> MTTKEFEDTWAYNTIGSPFPDNPVRVKGQQNMYVALWYKFGKPIHGRAWNDNGNVECSFPYNKVELTGARDLGGQIQILTATEQDPTEQFKKTGFWYEWRPYKDRVNDQLLQLVRCGQSTPV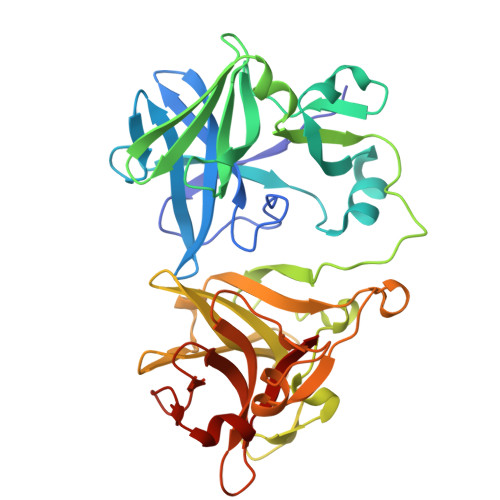IMKTKDGKDLLGYIDMSTEVAAVGVSGKSEQVAGGPIQDMLVLFRNVKAPPKGIKIYDDTWLDLKYRDPFPAARNPIAAGGRKVKSDDGTEMFQYVALWYEHGQPVFGRAYPDSADKTLANFGWGGQENAGAEIGSFQMLVVPDPDILGFEYKWIPYKEAKAGGPFKPLHVGECTPCLLKDANGTERLGNLHMGMEKATAGLAGKDSAVSGPAVGDFLVLCRN>[2x]MAHHHHHHGSKAYLVGLYTLTPTHPGSGTELGVVDQPIQRERHTGFPVIWGQSLKGVLRSYLKLVEKVDEEKINKIFGPPTEKAHEQAGLISVGDAKILFFPVRSLKGVYAYVTSPLVLNRFKRDLELAGVKNFQTEIPELTDTAIASEEITVDNKVILEEFAILIQKDDKGILESVVKAIEQAFGNEMAEKIKG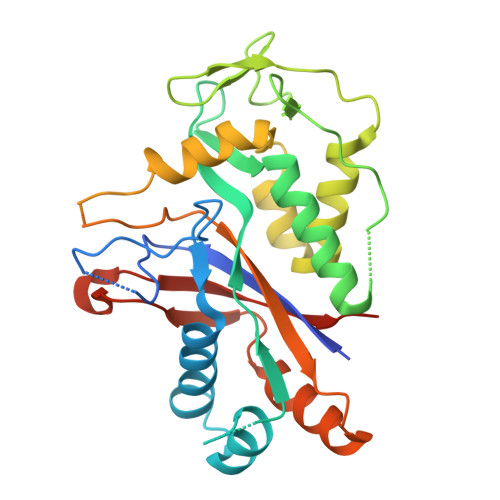RIAIIPDDVFRDLVELSTEIVARIRINAETGTVETGGLWYEEYIPSDTLFYSLILVTPRAKDNDMALIKEVLGKINGKYLQIGGNETVGKGFVKVTLKEVTNNGGTHAK> MVYHLFERICNPDNFKLSGEAARVRTLIAAGFSKEEAEQVAWLQNHQVNGKILGLFTGGFALYCCNNYFHYFERYFPRLRYQPFTKFLAQAATVYFFFKIGDY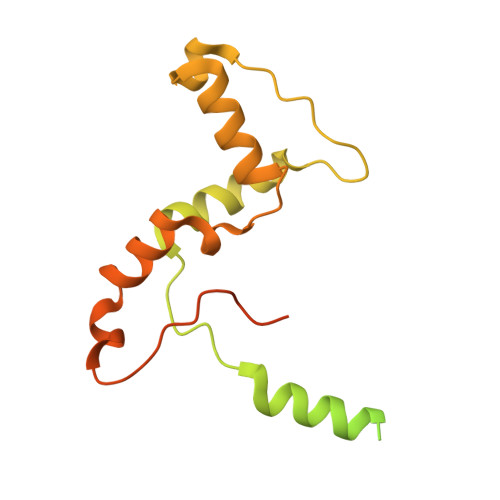YFTSRRYGSNDARMNGLMYSNTYYSTNKEALIQNFEPLNRKFTEEEVEQFLRNEGRSQEEKRNWIYNPHIHGSTEGEWKADIHEKFDSGKAPWEREHVKAKILETNKAKIDAGEEIQLKPFKTLNHLDKTGLLHRLHPFIWTNNWTLLG> MASGSCQGCEEDEETLKKLIVRLNNVQEGKQIETLVQILEDLLVFTYSEHASKLFQGKNIHVPLLIVLDSYMRVASVQQVGWSLLCKLIEVCPGTMQSLMGPQDVGNDWEVLGVHQLILKMLTVHNASVNLSVIGLKTLDLLLTSGKITLLILDEESDIFMLIFDAMHSFPANDEVQKLGCKALHVLFERVSEEQLTEFVENKDYMILLSALTNFKDEEEIVLHVLHCLHSLAIPCNNVEVLMSGNVRCYNIVVEAMKAFPMSERIQEVSCCLLHRLTLGNFFNILVLNEVHEFVVKAVQQYPENAALQISALSCLALLTETIFLNQDLEEKNENQENDDEGEEDKLFWLEACYKALTWHRKNKHVQEAACWALNNLLMYQNSLHEKIGDEDGHFPAHREVMLSMLMHSSSKEVFQASANALSTLLEQNVNFRKILLSKGIHLNVLELMQKHIHSPEVAESGCKMLNHLFEGSNTSLDIMAAVVPKILTVMKRHETSLPVQLEALRAILHFIVPGMPEESREDTEFHHKLNMVKKQCFKNDIHKLVLAALNRFIGNPGIQKCGLKVISSIVHFPDALEMLSLEGAMDSVLHTLQMYPDDQEIQCLGLSLIGYLITKKNVFIGTGHLLAKILVSSLYRFKDVAEIQTKGFQTILAILKLSASFSKLLVHHSFDLVIFHQMSSNIMEQKDQQFLNLCCKCFAKVAMDDYLKNVMLERACDQNNSIMVECLLLLGADANQAKEGSSLICQVCEKESSPKLVELLLNSGSREQDVRKALTISIGKGDSQIISLLLRRLALDVANNSICLGGFCIGKVEPSWLGPLFPDKTSNLRKQTNIASTLARMVIRYQMKSAVEEGTASGSDGNFSEDVLSKFDEWTFIPDSSMDSVFAQSDDLDSEGSEGSFLVKKKSNSISVGEFYRDAVLQRCSPNLQRHSNSLGPIFDHEDLLKRKRKILSSDDSLRSSKLQSHMRHSDSISSLASEREYITSLDLSANELRDIDALSQKCCISVHLEHLEKLELHQNALTSFPQQLCETLKSLTHLDLHSNKFTSFPSYLLKMSCIANLDVSRNDIGPSVVLDPTVKCPTLKQFNLSYNQLSFVPENLTDVVEKLEQLILEGNKISGICSPLRLKELKILNLSKNHISSLSENFLEACPKVESFSARMNFLAAMPFLPPSMTILKLSQNKFSCIPEAILNLPHLRSLDMSSNDIQYLPGPAHWKSLNLRELLFSHNQISILDLSEKAYLWSRVEKLHLSHNKLKEIPPEIGCLENLTSLDVSYNLELRSFPNEMGKLSKIWDLPLDELHLNFDFKHIGCKAKDIIRFLQQRLKKAVPYNRMKLMIVGNTGSGKTTLLQQLMKTKKSDLGMQSATVGIDVKDWPIQIRDKRKRDLVLNVWDFAGREEFYSTHPHFMTQRALYLAVYDLSKGQAEVDAMKPWLFNIKARASSSPVILVGTHLDVSDEKQRKACMSKITKELLNKRGFPAIRDYHFVNATEESDALAKLRKTIINESLNFKIRDQLVVGQLIPDCYVELEKIILSERKNVPIEFPVIDRKRLLQLVRENQLQLDENELPHAVHFLNESGVLLHFQDPALQLSDLYFVEPKWLCKIMAQILTVKVEGCPKHPKGIISRRDVEKFLSKKRKFPKNYMTQYFKLLEKFQIALPIGEEYLLVPSSLSDHRPVIELPHCENSEIIIRLYEMPYFPMGFWSRLINRLLEISPYMLSGRERALRPNRMYWRQGIYLNWSPEAYCLVGSEVLDNHPESFLKITVPSCRKGCILLGQVVDHIDSLMEEWFPGLLEIDICGEGETLLKKWALYSFNDGEEHQKILLDDLMKKAEEGDLLVNPDQPRLTIPISQIAPDLILADLPRNIMLNNDELEFEQAPEFLLGDGSFGSVYRAAYEGEEVAVKIFNKHTSLRLLRQELVVLCHLHHPSLISLLAAGIRPRMLVMELASKGSLDRLLQQDKASLTRTLQHRIALHVADGLRYLHSAMIIYRDLKPHNVLLFTLYPNAAIIAKIADYSIAQYCCRMGIKTSEGTPGFRAPEVARGNVIYNQQADVYSFGLLLYDILTTGGRIVEGLKFPNEFDELEIQGKLPDPVKEYGCAPWPMVEKLIKQCLKENPQERPTSAQVFDI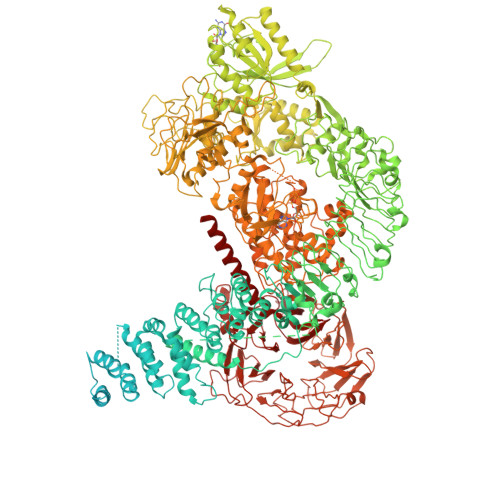LNSAELVCLTRRILLPKNVIVECMVATHHNSRNASIWLGCGHTDRGQLSFLDLNTEGYTSEEVADSRILCLALVHLPVEKESWIVSGTQSGTLLVINTEDGKKRHTLEKMTDSVTCLYCNSFSKQSKQKNFLLVGTADGKLAIFEDKTVKLKGAAPLKILNIGNVSTPLMCLSESTNSTERNVMWGGCGTKIFSFSNDFTIQKLIETRTSQLFSYAAFSDSNIITVVVDTALYIAKQNSPVVEVWDKKTEKLCGLIDCVHFLREVTVKENKESKHKMSYSGRVKTLCLQKNTALWIGTGGGHILLLDLSTRRLIRVIYNFCNSVRVMMTAQLGSLKNVMLVLGYNRKNTEGTQKQKEIQSCLTVWDINLPHEVQNLEKHIEVRKELAEKMRRTSVE>[2x]GPGHMVVKFSYMWTINNFSFCREEMGEVIKSSTFSSGANDKLKWCLRVNPKGLDEESKDYLSLYLLLVSCPKSEVRAKFKFSILNAKGEETKAMESQRAYRFVQGKDWGFKKFIRRGFLLDEANGLLPDDKLTLFCEVSVVQD;>[2x]AEGTVSSSTDALPCI

The SPOP gene encodes a substrate-binding adaptor subunit of the CULLIN3 (CUL3)-RING box 1 (RBX1) E3 ubiquitin ligase (CRL) complex. Geminin and its binding partner Cdt1 are essential for the regulation of DNA replication. Here we show that the CULLIN3 E3 ubiquitin ligase adaptor protein SPOP binds Geminin at endogenous level and regulates DNA replication. SPOP promotes K27-linked non-degradative poly-ubiquitination of Geminin at lysine residues 100 and 127.

Proteins bound by SPOP usually harbor a SPOP-binding consensus sequence (SBC, Φ-π-S-S/T-S/T where Φ is a nonpolar residue and π is a polar residue). The C-terminal segment 199VSSST203 is the only putative SBC motif in Geminin. We also determined the X-ray crystal structure of SPOP-MATH domain in complex with the Geminin peptide 195AEGTVSSSTDAKPCI209 to a resolution of 3.4 Å. There are two copies of SPOP-Geminin complex in the asymmetric unit. The Geminin peptide electron density is detectable for each complex, within which we could fit nine Geminin residues from Glu196 to Asp204. Consistent with our NMR data, the peptide lies in a shallow groove across SPOP surface. The binding mode in SPOP-Geminin is similar to those in crystal structures of SPOP complexed with other peptides. Geminin Val199 sits in a hydrophobic pocket formed by SPOP Phe102, Tyr123, Trp131, and Phe133, while Geminin Ser200, Ser201, and Ser202 probably participate in a network of intermolecular hydrogen bonds with SPOP residues Lys129, Asp130, Gly132, and Lys134. The Geminin 199VSSST203 motif contributes 8 out of 9 putative intermolecular hydrogen bonds between SPOP and Geminin. In contrast, there were almost no changes in the 1H-15N HSQC spectrum of SPOP MATH upon addition of Geminin SBC-alanine mutant peptide, demonstrating that the SBC motif 199VSSST203 is essential for SPOP-Geminin interaction.>APASLLPPAPEHSPPSSPLTQPPEGPKFPRVKNWEVGSITYDTLSAQAQQDGPCTPRRCLGSLVFPRKLQGRPSPGPPAPEQLLSQARDFINQYYSSIKRSGSQAHEQRLQEVEAEVAATGTYQLRESELVFGAKQAWRNAPRCVGRIQWGKLQVFDARDCRSAQEMFTYICNHIKYATNRGNLRSAITVFPQRCPGRGDFRIWNSQLVRYAGYRQQDGSVRGDPANVEITELCIQHGWTPGNGRFDVLPLLLQAPDEPPELFLLPPELVLEVPLEHPTLEWFAALGLRWYALPAVSNMLLEIGGLEFPAAPFSGWYMSTQIGTRNLCDPHRYNILEDVAVCMDLDTRTTSSLWKDKAAVEINVAVLHSYQLAKVTIVDHHAATASFMKHLENEQKARGGCPADWAWIVPPISGSLTPVFHQEMVNYFLSPAFRYQPDPW[4x]

Nitric oxide (NO) is an important signaling molecule critical in the cardiovascular, neuronal, and immune systems. The enzyme responsible for generating NO is nitric oxide synthase (NOS), a P450-like heme thiolate enzyme that oxidizes l-arginine to NO and L-citrulline. Humans and other mammals express three different NOS isoforms: endothelial NOS (eNOS), neuronal NOS (nNOS), and inducible NOS (iNOS). nNOS is an important therapeutic target since the overproduction of NO by nNOS in the brain is associated with a number of neurodegenerative diseases. Thus, nNOS is an attractive target for therapeutic intervention. In our efforts to develop inhibitors selective for neuronal nitric oxide synthase (nNOS) over endothelial nitric oxide synthase (eNOS), we found that nNOS can undergo conformational changes in response to inhibitor binding that does not readily occur in eNOS. Here, we used a combination of crystallography, mutagenesis, and computational methods to better understand the structural basis for these differences in NOS inhibitor binding.

We asked the questions, how can the inhibitor displace BH4, and does the inhibitor displacing BH4 in hnNOS bind synergistically or independently from the inhibitor bound in the active site? To explore these questions, we “knocked out” the active site inhibitor binding by mutating the active site Glu to Gln in both hnNOS and heNOS to generate hnNOS E597Q and heNOS E361Q. 4 binds in neither the active site nor the BH4 site in these hnNOS and heNOS mutants. This result indicates that the binding of two inhibitor molecules is synergistic and that one molecule must first bind in the active site before a second molecule binds in the BH4 pocket. In this study, we also found that the binding of a second inhibitor molecule in the BH4 pocket first requires the binding of the inhibitor to the active site.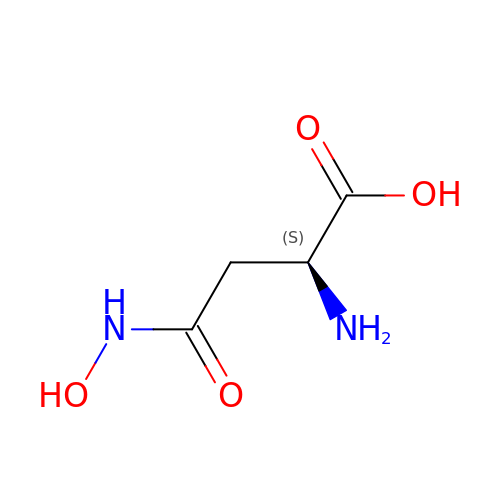N-hydroxy-L-asparagine | C4 H8 N2 O4 | ZBYVTTSIVDYQSO-REOHCLBHSA-N> GSHMEAVQNRIVEAAERVPGVRGVIHLRARYVGQDIWADMIIGVDPENTVEQAHEICEAVQAAVCGKIRRIESLHVSADAREIGD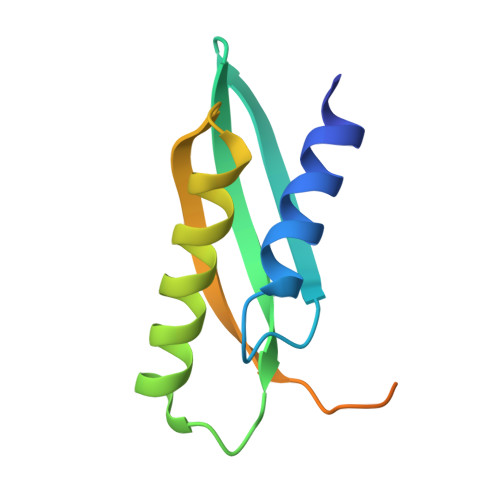TTKPSFSDQPLSFDEVMLSKVDN>[2x]MGSDKIHHHHHHMQVPKVTLNNGVEMPILGYGVFQIPPEKTEECVYEAIKVGYRLIDTAASYMNEEGVGRAIKRAIDEGIVRREELFVTTKLWVSDVGYESTKKAFEKSLKKLQLEYIDLYLIHQPFGDVHCAWKAMEEMYKDGLVRAIGVSNFYPDRLMDLMVHHEIVPAVNQIEIHP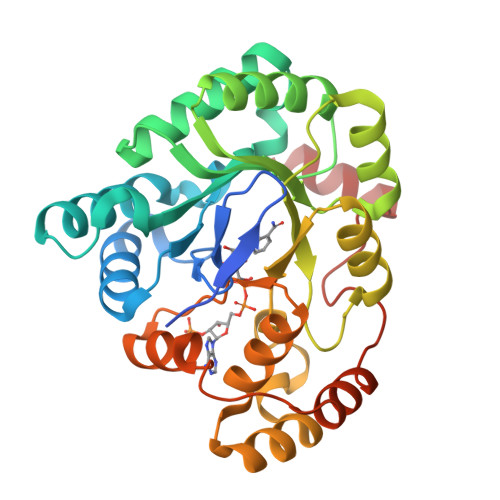FYQRQEEIEFMRNYNIQPEAWGPFAEGRKNIFQNGVLRSIAEKYGKTVAQVILRWLTQKGIVAIPKTVRRERMKENISIFDFELTQEDMEKIATLDEGQSAFFSHRDPEVVKWICSLKR> EYERRIAARFTTFDQDGNGHIDRSDFSGAAKAMLAEFGVAARSDRGQALYGGAEALWQGLAGIADRDGDQRITREEFVTGAVKRLRDKPDRFAEMARPFLHAALGVADTDGDGA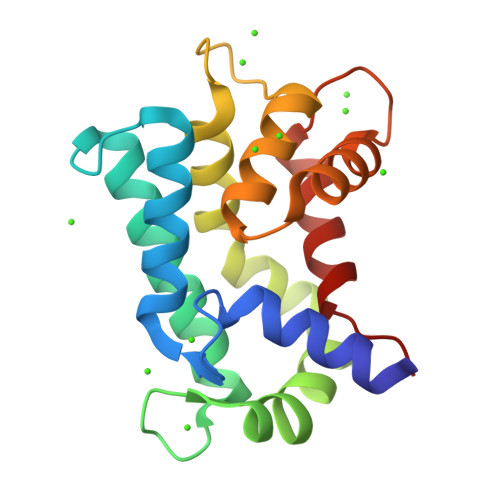VTVADTARALTAFGVPEDLARQAAAALDTDGDGKVGETEIVPAFARYFTVPA Arginase (Arginine amidinase; EC 3.5.3.1) is one of the enzymes involved in the final step of the urea cycle. In the reported arginase structures, their active sites contain a binuclear manganese cluster that is coordinated by one or two water molecules and two histidine and four aspartate residues from three conserved sequence motifs of GGDHS, DAHXD, and SXDXDXDP. Among them, the ZMO0432 gene product annotated as an arginase (zmARG) has the three sequence motifs found in arginase proteins. In this study, we have shown that zmARG catalyzed the arginine-hydrolyzing activity in a manganese ion-dependent manner and the dimeric state is formed by a novel helix-swapping manner.

In order to get the structural background for the enzymatic activity of zmARG, its crystal structure was determined at a resolution of 1.65 Å. The refined structure shows four molecules in the asymmetric unit of the C2 space group. The elucidated crystal structure of zmARG shows a common arginase fold with a protruding α-helix at the C-terminus that mediates a dimerization of the protein. The refined zmARG structure has shown two strong spherical electron densities in the pocket of each α/β hydrolase fold, which were modeled as zinc ions, based on the X-ray absorption near edge structure (XANES) and a fluorescence scan. The deep pocket with the two metal-binding sites of zmARG is lined with residues of the arginase-forming conserved sequence motifs of 89GGDCL93, 116DSHPD120, and 210HIDLDVLDP218. The first zinc ion is coordinated with five atoms of Sγ of Cys92, three Oδs of Asp116, Asp120, and Asp212, and the metal-bridging water molecule, which forms a distorted trigonal bipyramid configuration. On the other hand, the second zinc ion is hexa-coordinated with four Oδ atoms of Asp116, Asp212, and Asp214 (bidentate), Nε atom of His118, and the metal-bridging water molecule, and forms an octahedral geometry. Furthermore, the first zinc ion of zmARG forms a trigonal bipyramid by five ligands while the second one is octahedrally coordinated by six ligands, which is different from two metal ions of an octahedral geometry in other arginases. Notably, the C-terminal tail including the α10-helix (Trp273-Glu284) of each protomer ptotrudes outside from the globular α/β hydrolase fold and interacts with the open hydrophobic pocket on the surface formed by the two α-helices (α1 and α9) and the central β-sheet of the neighboring molecule. Based on the assays with deprivation of the metal ions taken from the expression host and loading metal ions into the active site, it can be argued that zmARG is also a manganese ion-dependent arginase like other arginases.

>MSSINKPLRLIFPQWQGGDNPPYYLGSQLLAWLSPDPKGAVEEVPVPKPTGEPLQEENGIVGRSILIDQLSEARQLIEKHTPDSLVVLGGDCLVSLAPFSWLLEKYKDKLGILWIDSHPDVQTPKEYKNAHAHVLGELMGNGDSDFTRTVKHPVSPQKIMIAGIHDPLPYEANFISEHKIQTCSPEQVRSGAQPVLDWIKNEKIEYLAIHIDLDVLDPHNFRSVLFAKPGRGQHDFGDVAEGKLNIPDVVKLANQAASISKAVGLTIAEHLPWDALNLKNMLEELPLIGK[4x]> WGKEGHEIICKIAQTRLDETAAKAVKELLPESAEGDLSSLCLWADRVKFRYHWSSPLHYINTPDACSYQYNRDCKDESGEKGRCVAG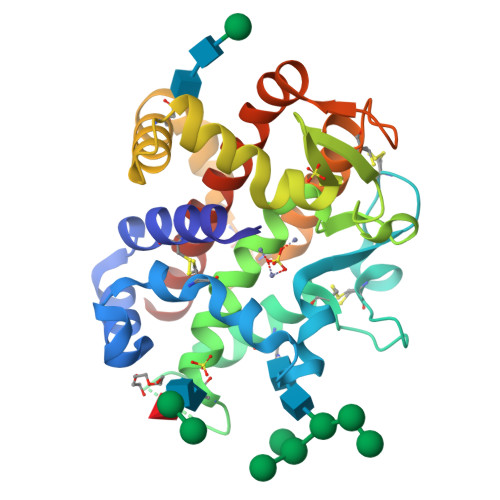AIYNYTTQLLSYKTAASSQSQYNLTEALLFVSHFMGDIHQPLHVSYASDKGGNTIEVHWYTRKANLHHIWDSNIIETAEADLYNSALEGMVDALKKNITTEWADQVKRWETCTKKTACPDIYASEGIQAACDWAYKGVTEGDTLEDEYFYSRLPIVYQRLAQGGVRLAATLNRIFGHHHHHH> MRIDPFKLAHWMNARKYTAAQTADLAGLPLDDLRRLLGDEANEPDPAAATALAEALSVEPSQLAADAHRNLTVVHKSAEEMHASRRPIQRDGIHFYNYYTLAAPEGRVAPVVLDILCPSDRLPALNNGHLEPAITVNLGPGDINGRWGEEITPQTWRVLHANHGGDRWITGDS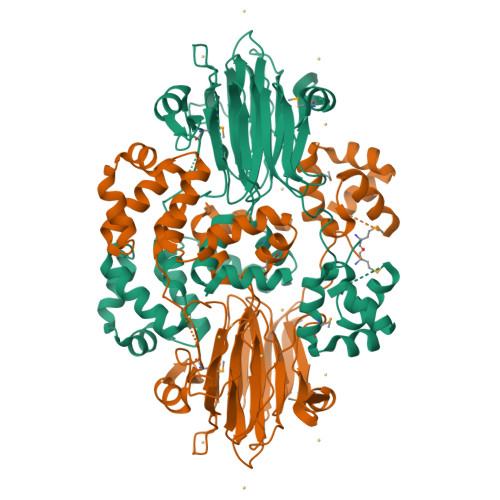YVEPSYCPHSYSLAGDAPARIVSYTAQSNISPLMTEANNWSTGAFEEALKALSGKVSAGSVLDLFLARRAHTRTSAAEAAGVPPADLEAALRSPASETGLTVLRTLGRALGFDYRVLLPADDQHDGVGKTWTTIEDSRRSRRTFGTYEAASMASAAHLPDLVGSFLRVDADGRGADLIDHAENHYVVTEGRLTLEWDGPDGPASVELEPDGSAWTGPFVRHRWHGTGTVLKFGSGAHLGYQDWLELTNTFEPAATLRRGRRDLAGWGYDN> MHHHHHHQIGWRREGIKYRRNELFLDVLESVNLLMSPQGQVLSAHVSGRVVMKSYLSGMPECKFGMNDKIVIEKQGKGTADETSKSGKQSIAIDDCTFHQCVRLSKFDSERSISFIPPDGEFELMRYRTTKDIILPFRVIPLVREVGRTKLEVKVVIKSNFKPSLLAQKIEVRIPTPLNTSGVQVICMKGKAKYKASENAIVWKIKRMAGMKESQISAEIELLPTNDKKKWARPPISMNFEVPF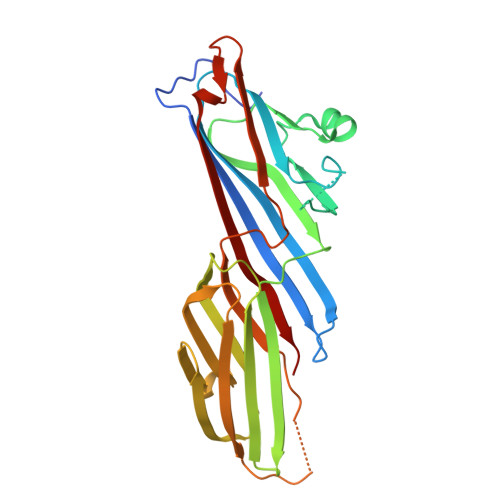APSGLKVRYLKVFEPKLNYSDHDVIKWVRYIGRSGIYETRC>AMADIGSDVASLRQQVEA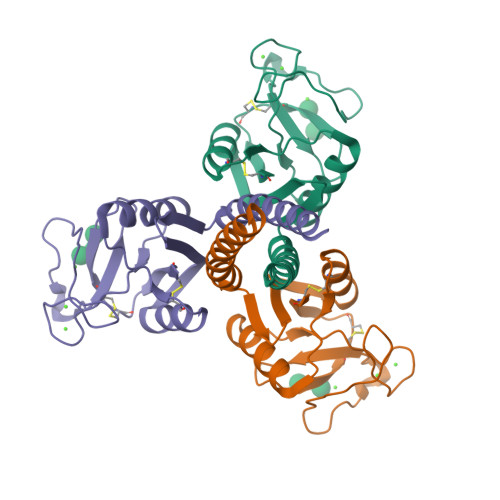LQGQVQHLQAAFSQYKKVELFPNGQSVGEKIFKTAGFVKPFTEAQLLCTQAGGQLASPRSAAENAALQQLVVAKNEAAFLSMTDSKTEGKFTYPTGESLVYSNWAPGEPNDDGGSEDCVEIFTNGKWNDRACGEKRLVVCEF[3x]> MGVAL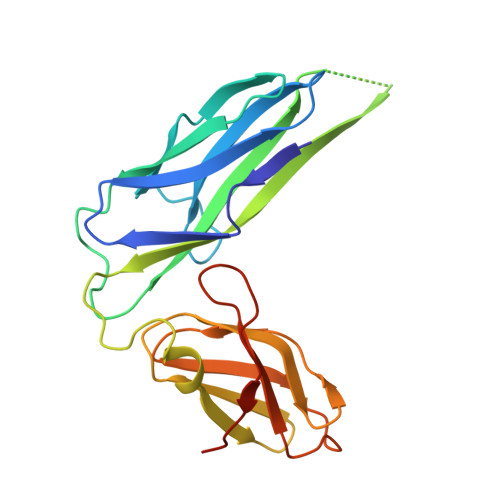GATRVIYPAGQKQEQLAVTNNDENSTYLIQSWVENADGVKDGRFIVTPPLFAMKGKKENTLRILDATNNQLPQDRESLFWMNVKAIPSMDKSKLTENTLQLAIISRIKLYYRPAKLALPPDQAAEKLRFRRSANSLTLINPTPYYLTVTELNAGTRVLENALVPPMGESTVKLPSDAGSNITYRTINDYGALTPKMTGVMEHHHHHH> GPHMLELTKEQLYQQAMEEAAWHHMPHPSDSERIRQYLPRNPCPTPPYHHQMPPPHSDTVEFYQRLSTETLFFIFYYLEGTKAQYLAAKALKKQSWRFHTKYMMWFQ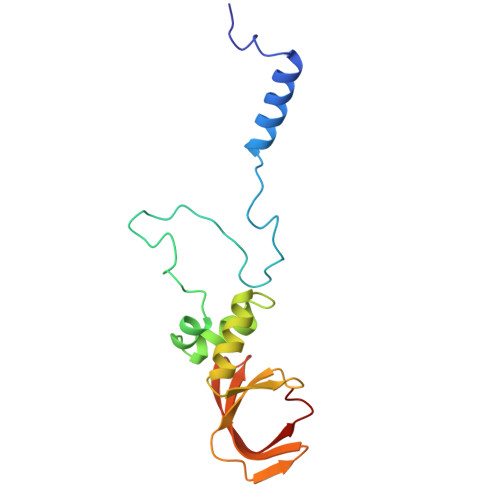RHEEPKTITDEFEQGTYIYFDYEKWGQRKKEGFTFEYRYLE1-O-OCTYL-2-HEPTYLPHOSPHONYL-SN-GLYCERO-3-PHOSPHOETHANOLAMINE 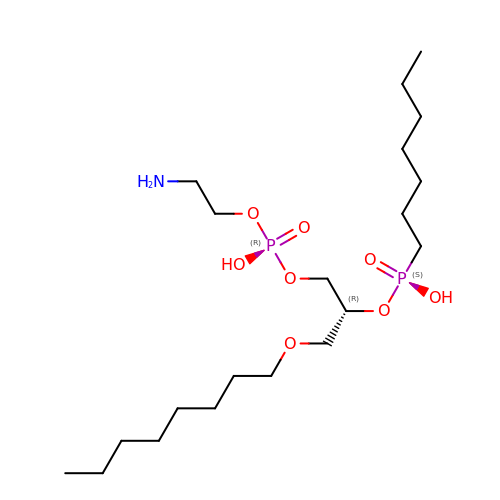| C20 H45 N O8 P2 | RCCNUBYROFOKAU-HXUWFJFHSA-N> KESAAAKFERQHMDSGNSP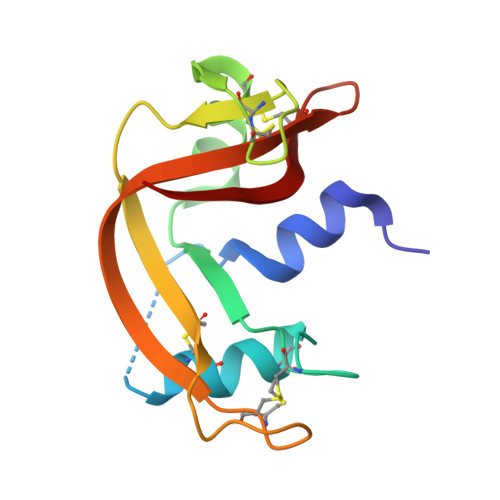SSSSNYCNLMMCCRKMTQGKCKPVNTFVHESLADVKAVCSQKKVTCKNGQTNCYQSKSTMRITDCRETGSSKYPNCAYKTTQVEKHIIVACGGKPSVPVHFDASV> HLEVVKLLLEHGA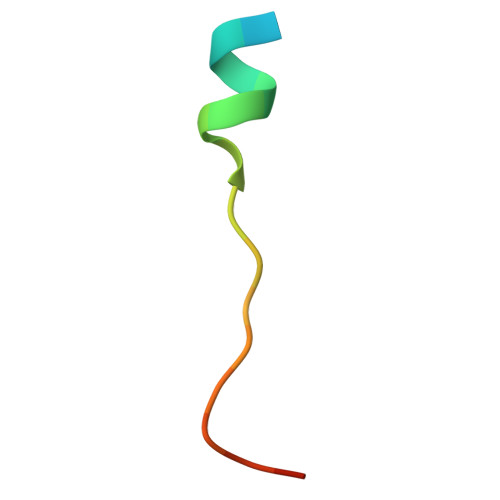DVSAQDK>MASLTVKAYLLGKEDAAREIRRFSFCCSPEPEAEAEAAAGPGPCERLLSRVAALFPALRPGGFQAHYRDEDGDLVAFSSDEELTMAMSYVKDDIFRIYIKEKKECR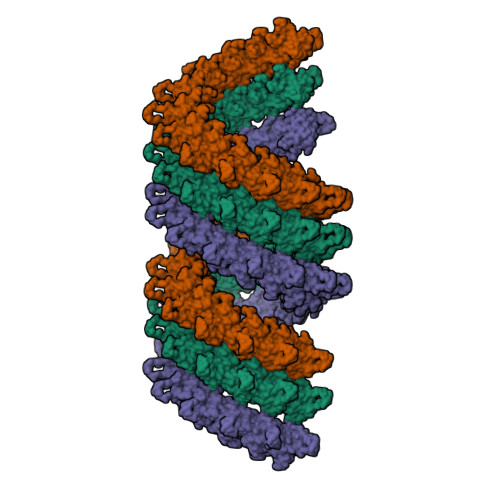RDHRPPCAQEAPRNMV[3x]The hammerhead ribozyme, since its discovery in satellite virus RNA genomes, has been a central focus of experiments designed to correlate RNA structure with RNA catalysis, as it is a comparatively small RNA whose biochemistry has been intensively investigated using a wide variety of approaches. The most well-characterized member of the first class of natural hammerheads occurs within the satellite RNA of the tobacco ringspot virus (sTRSV), which is also the first hammerhead ribozyme discovered. Instead of inactivating the nucleophile via methylation, as was done with the Schistosome hammerhead, the cleavage reaction in the case of the sTRSV hammerhead has been greatly decelerated with a G12A enzyme active site variant that lowers the pKa of the purine general base in the cleavage reaction from approximately 9.5 to approximately 3.5, which, assuming the observed log-linear rate dependence on pH, potentially represents an approximately 106-fold decrease of the reaction rate. By greatly slowing the reaction, the hammerhead RNA crystallizes prior to cleavage, but remains active in the crystal and slowly cleaves.

Refinement of a hypothetically uncleaved structure using the 2.2 Å resolution cleavage product dataset, obtained from the crystals allowed to age, revealed unique and significant (>3 σ) negative difference Fourier peaks positioned directly on the O5′ atoms of A1.1 of each molecule of the hypothetically uncleaved model (without noncrystallographic symmetry averaging applied), in addition to clear breaks in the sigma-A–weighted 2Fo-Fc maps at the same locations, thus demonstrating that the substrate RNA is predominantly in the cleaved state. The negative difference Fourier peak on molecule 1 is slightly more pronounced, and subsequent refinement of the structure in which a 2′,3′-cyclic phosphate was added to C17, and the phosphate linking it to A-1.1 was replaced with a terminal 5′-OH, provided a much better fit to the observed electron density. Molecule 1 appears to be completely cleaved, whereas a small amount of molecule 2 may remain in the uncleaved form. The cleaved structure reveals several interactions potentially relevant to the catalytic mechanism. In molecule 1 of the cleavage product structure, two Mg2+ ions appear to interact with the scissile phosphate, which is in the 2′,3′-cyclic form. In addition, the 2′-OH of G8, previously implicated as possibly the acid catalyst, makes a hydrogen bond to the more proximal nonbridging phosphate oxygen of the cyclic phosphate. N1 and N6 of A9 are also positioned about 4.5 Å from the same nonbridging cyclic phosphate oxygen atom, as is the Mg2+ ion bound to A9 phosphate.

>GGGAGCCCUGUC[2x];>[2x]ACCGGAUGUGCUUUCCGGUCUGAUGAGUCCGUGAGGACAAAACAGGGCUCCCGAAUU> MTQSLFQPITLGALTLKNRIVMPPLTRSRASQPG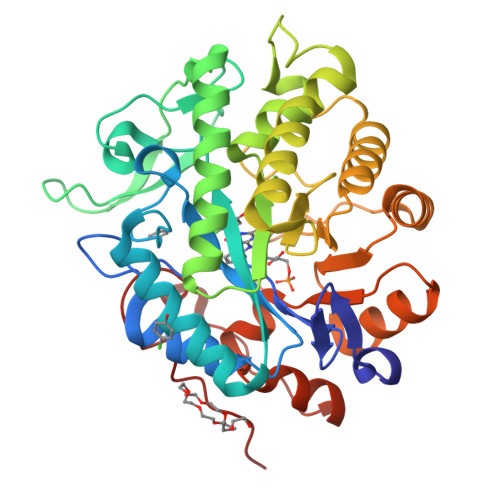DVANHMMAIYYAQRASAGLIVSEGTQISPTAKGYAWTPGIYTPEQIAGWRIVTEAVHAKGCAIFAQLWHVGRVTHPDNIDGQQPISSSTLKAENVKVFVDNGSDEPGFVDVAVPRAMTKADIAQVIADYRQAALNAMEAGFDGIELHAANGYLINQFIDSEANNRSDEYGGSLENRLRFLDEVVAALVDAIGAERVGVRLAPLTTLNGTVDADPILTYTAAAALLNKHRIVYLHIAEVDWDDAPDTPVSFKRALREAYQGVLIYAGRYNAEKAEQAINDGLADMIGFGRPFIANPDLPERLRHGYPLAEHVPATLFGGGEKGLTDYPTYQA Thymine DNA glycosylase (TDG) is a base excision repair (BER) enzyme that acts on derivatives of 5-methylcytosine (mC) arising from deamination or oxidation. TDG excises thymine from G·T mispairs, an activity that is needed to protect against C→T transition mutations caused by deamination of mC to T. It also plays an essential role in active DNA demethylation, which likely accounts for findings that its depletion in mice causes embryonic lethality. One established pathway for active DNA demethylation involves TDG excision of 5-formylcytosine or 5-carboxylcytosine, oxidation derivatives of mC generated by TET (ten–eleven translocation) enzymes. To address this problem, we developed improved crystallization conditions for TDG and solved high-resolution (up to 1.45 Å) structures of product complexes generated from substrates including G·hmU, G·T, G·U, G·fC and G·caC.

To rule out the possibility that acetate displaces the excised base in the product complex, we grew crystals of a TDGcat product complex, generated from a G·U substrate, using mother liquor that did not contain acetate and solved a structure at 1.75 Å resolution. The electron density demonstrates that the active site does not contain acetate or the excised uracil base. Rather, it contains only water molecules and the abasic sugar. Moreover, crystals grown under acetate-free conditions yield structures of the E·P complex that contain only water molecules in the active site. Interestingly, our new structures indicate that absence of the excised base (or acetate) in the active site impacts the equilibrium between the two potential anomeric forms of the abasic sugar produced by TDG. However, for those crystallized under acetate-free conditions, the abasic sugar exists in a roughly equal mix of α and β anomers, each forming different interactions involving C1’-OH. The β anomer contacts several ordered water molecules in the active-site, while the α anomer contacts the Oδ of Asn140, the side chain that coordinates the putative water nucleophile in the E·S complex. Our findings show that dissociation of the excised base is required for TDG binding to the β anomer of the abasic sugar.

> GSHMASFNGVSEAELLTKTLPDILTFNLDIVIIGINPGLMAAYKGHHYPGPGNHFWKCLFMSGLSEVQLNHMDDHTLPGKYGIGFTNMVERTTPGSKDLSSKEFREGGRILVQKLQKYQPRIAVFNGKCIYEIFSKEVFGVKVKNLEFGLQPHKIPDTETLCYVMPSSSARCAQFPRAQDKVHYYIKLKDLRDQLKGIERNMDV BENZYL 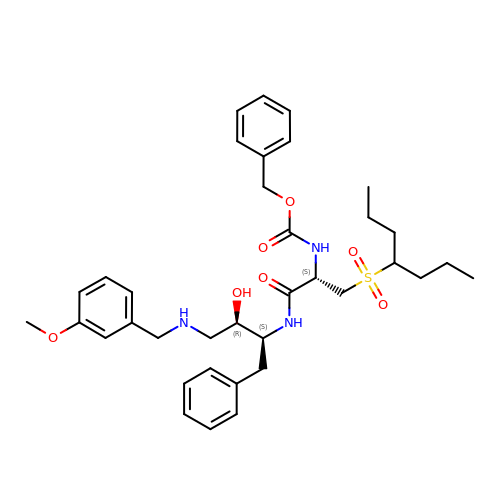[(1S)-2-({(1S,2R)-1-BENZYL-2-HYDROXY-3-[(3-METHOXYBENZYL)AMINO]PROPYL}AMINO)-2-OXO-1-{[(1-PROPYLBUTYL)SULFONYL]METHYL}ETHYL]CARBAMATE | C36 H49 N3 O7 S | FJYALDRNDKNYKU-LBFZIJHGSA-N>MELIRIAMRKDLENDKSLMSKWAAVAGLKNPNPLYDFLNHDGKTFSEFNSIVNIVKTHYPDQEYELMENYCLLLDPNTKAARSALEYADANSFNTLTDKLVEKMSIASNLKSKEYGKIYEIHRKLSRGEIDVLEASKNIGKYRIKTDEMNIFSKMIPMYDYLSKGNFSPMKSLLKQIDLNDIKENNYLKKSFETRIYVLLSNIYLNENELELSRKYAEKAIKSTDTKRFLVFSYLTIGTSYIFSDYALSKQNYLSGYEIAKGNSVFEEFFKRNLSFLNNFWNKENPWINYDSNAVTDVQEVIFELINQKKLERALTLLKSLERKKQNENDLGFHYYLEGLITNDKEAFYKSVEYFKLS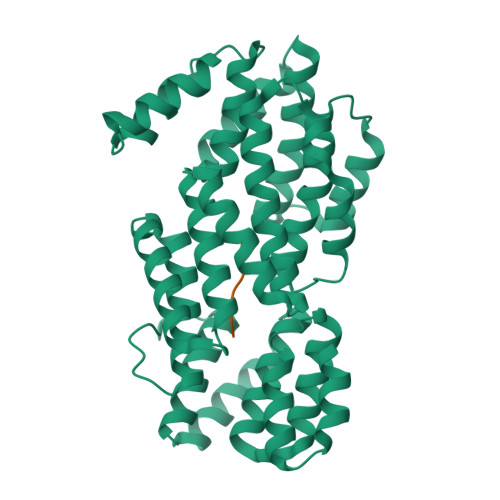QDKLFIKMPLIKLESLGENPRLLKIISM[4x];>[4x]GIVRGA> TLSILVAHDLQRVIGFENQLPWHLPNDLKNVKKLSTGHTLVMGRKTFESIGKPLPNRRNVVLTSDTSFNVEGVDVIHSIEDIYQLPGHVFIFGGQTLYEE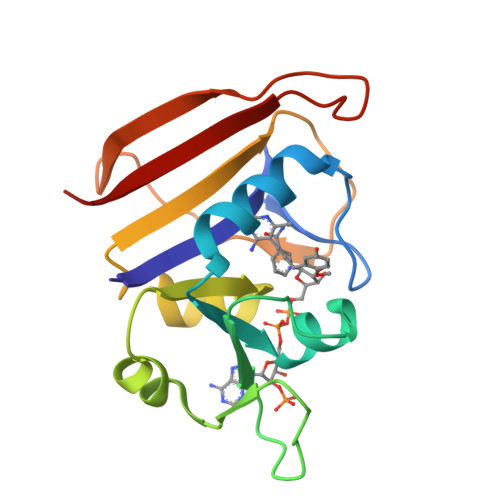MIDKVDDMYITVIEGKFRGDTFFPPYTFEDWEVASSVEGKLDEKNTIPHTFLHLIRK> CUGCUGGCUAAGGCCCGAA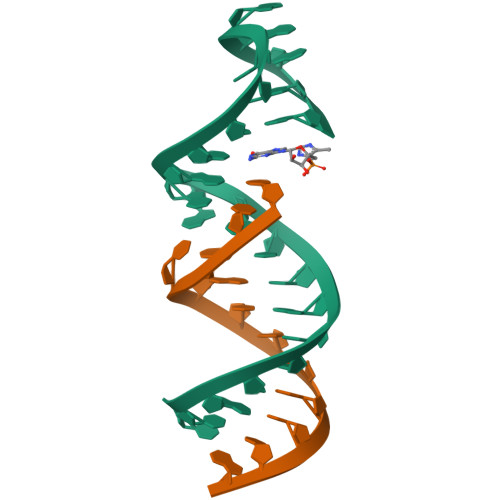AGG;> CUAUGCCUGCUG>[2x]MKQLTILGSTGSIGCSTLDVVRHNPEHFRVVALVAGKNVTRMVEQCLEFSPRYAVMDDEASAKLLKTMLQQQ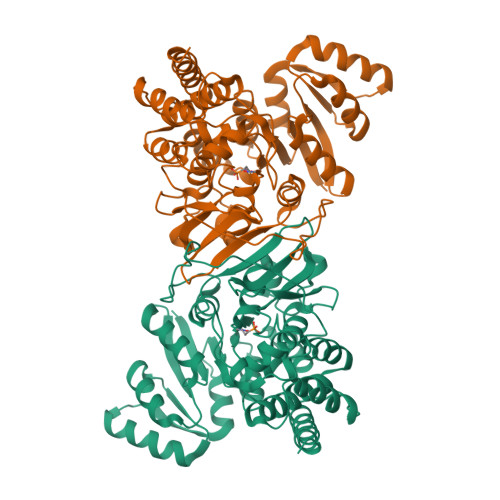GSRTEVLSGQQAACDMAALEDVDQVMAAIVGAAGLLPTLAAIRAGKTILLANKESLVTCGRLFMDAVKQSKAQLLPVDSEHNAIFQSLPQPIQHNLGYADLEQNGVVSILLTGSGGPFRETPLRDLATMTPDQACRHPNWSMGRKISVDSATMMNKGLEYIEARWLFNASASQMEVLIHPQSVIHSMVRYQDGSVLAQLGEPDMRTPIAHTMAWPNRVNSGVKPLDFCKLSALTFAAPDYDRYPCLKLAMEAFEQGQAATTALNAANEITVAAFLAQQIRFTDIAALNLSVLEKMDMREPQCVDDVLSVDANAREVARKEVMRLAS>[2x]MPKHEFSVDMTCGGCAEAVSRVLNKLGG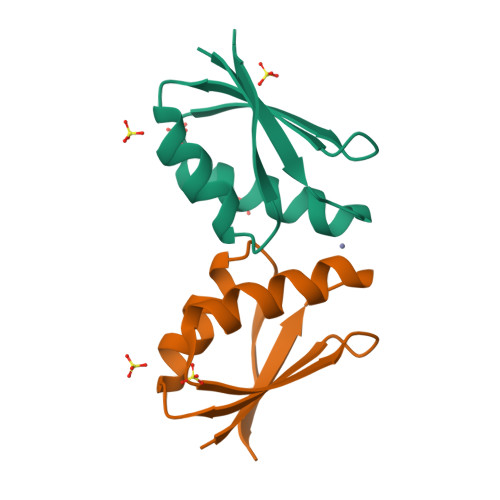VKYDIDLPNKKVCIESEHSMDTLLATLKKTGKTVSYLGLE>[4x]MTKQLPNLQVALDHSNLKGAITAAVSVGNEVDVIEAGTVCLLQVGSELVEVLRSLFPDKIIVADTKCADAGGTVAKNNAVRGADWMTCICSATIPTMKAARKAIEDINPDKGEIQVE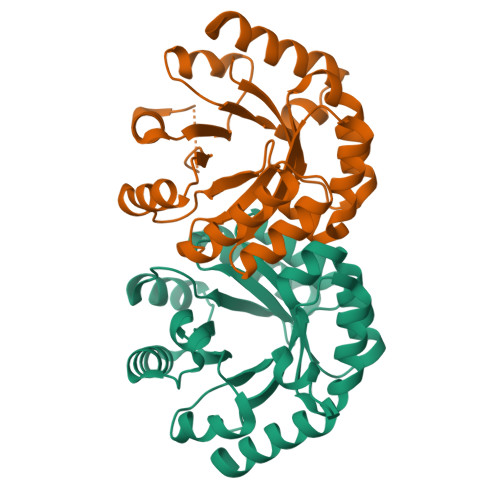LYGDWTYDQAQQWLDAGISQAIYHQSRDALLAGETWGEKDLNKVKKLIEMGFRVSVTGGLSVDTLKLFEGVDVFTFIAGRGITEAKNPAGAARAFKDEIKRIWG> GPKGEVISSGSKPLSPGPCLDIPSILSNKQFLAWGGVPLGRTQLQKLALRNNSASTTQHLRL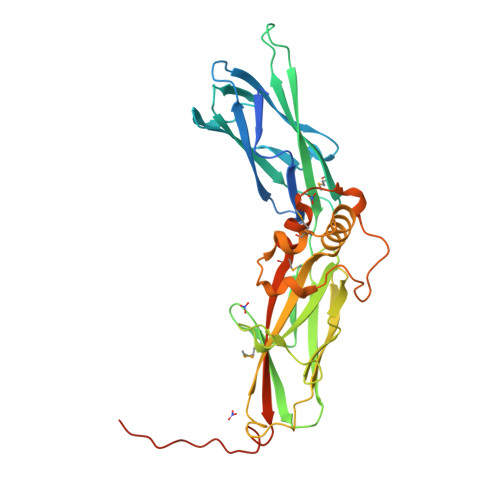LIRGQDQDCFQLQNTFGSEQRLTSNCEIRIHPKEDIFISVLFAPTRLSCMLARLEIKQLGNRSQPGIKFTIPLSGYGGTSNLILEGVKKLSDSYMVTVNGLVPGKESKIVFSVRNTGSRAAFVKAVGFKDSQKKVLLDPKVLRIFPDKFVLKERTQENVTLIYNPSDRGINNKTATELSTVYLFGGDEISRQQYRRALLHKPEMIKQILPEHSVLQNINFVEAFQDELLVTEVYDLPQRPNDVQLFYGSMCKIILSVIGEFRDCISSREFLQPSSKASLESTSDLGASGK> MDVVIAVGAPLTGPNAAFGAQIQKGAEQAAKDINAAGGINGEQIKIVLGDDVSDPKQGISVANKFVADGVKFVVGHANSGVSIPASEVYAENGILEITPAATNPVFTERGLWNTFRTCGRDDQQGGIAGK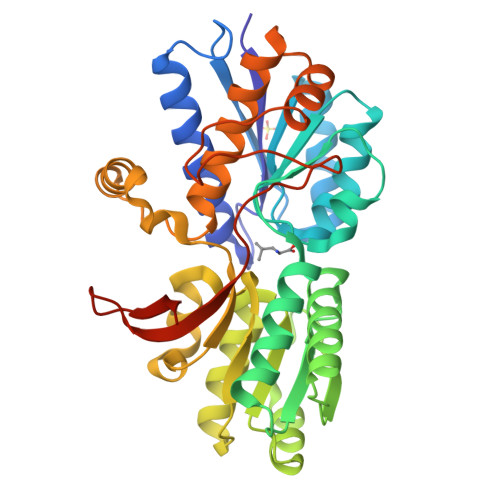YLADHFKDAKVAIIHDKTPYGQGLADETKKAANAAGVTEVMYEGVNVGDKDFSALISKMKEAGVSIIYWGGLHTEAGLIIRQAADQGLKAKLVSGDGIVSNELASIAGDAVEGTLNTFGPDPTLRPENKELVEKFKAAGFNPEAYTLYSYAAMQAIAGAAKAAGSVEPEKVAEALKKGSFPTALGEISFDEKGDPKLPGYVMYEWKKGPDGKFTYIQQGSHHHHHH>[6x]GMNRLRTSFQQTTGQISGHGKRNVGVLKTAFAAVADEMASDQYGTGAIIEPFEQKFADVLGMDDAVFFPSGTMAQQVALRIWSDETDNRTVAYHPLCHLEIHEQDGLKELHPIETILVGAADRLMTLDEIKALPDIACLLLELPQREIGGVAPAFSELETISRYCRERGIRLHLDGARLFEMLPYYEKTAAEIAGLFDSIYISFYKGLGGIAGAILAGPAAFCQTARIWKRRYGGDLISLYPYI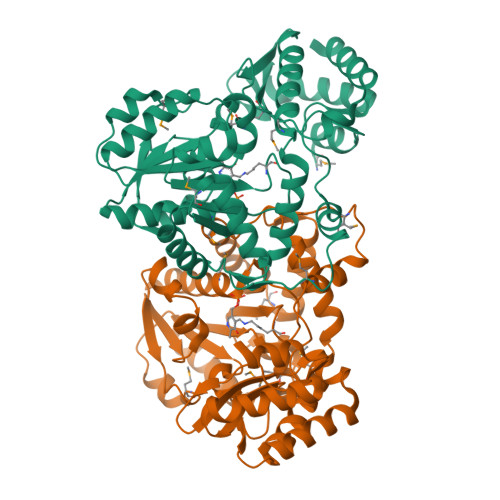VSADYYYELRKDRMGQYYEQAKQLAEQFNALPGVHTTPEVPVSNMFHLHFDGQAADISPKLEQVQEETGLGFVGYLVDKDGYCSTEISVGDAYGELDQQTRDAGFARLRQAFS>GIDPFTKMTRPSSDLTAFREHFAKAKHIAIITGAGVSAESGVPTFRGPGGFWRKWQAQDLATPEAFSRDPSLVWEFYHYRREVMRSKMPNPAHLAIAECEARLGQQGRSVVIITQNIDELHHRAGSKHVYEIHGSLFKTRCMSCGEVKANHKSPICPALDGKGAPDPNTKEARIPVELLPRCERKSCNGLLRPHVVWFGETLDSDILTAVERELEKCDLCLVVGTSSIVYPAAMFAPQVASRGVPVAEFNMECTPATQRFK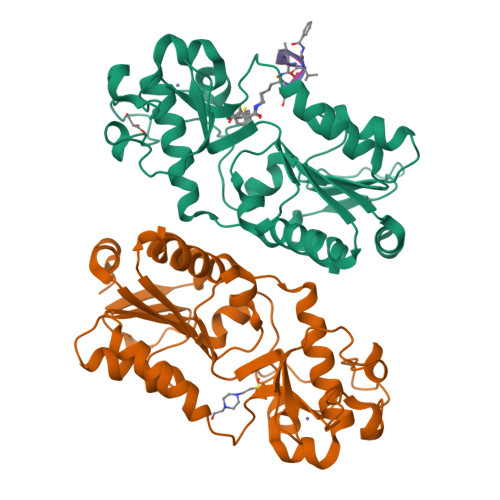YHFEGPCGSTLPPALERHESEAV[2x]~{tert}-butyl ~{N}-[(2~{S})-1-[(2~{S},4~{R})-2-[[(1~{R},2~{R})-1-(cyclopropylsulfonylcarbamoyl)-2-ethyl-cyclopropyl]carbamoyl]-4-(3-ethyl-7-methoxy-quinoxalin-2-yl)oxy-pyrrolidin-1-yl]-3,3-dimethyl-1-oxidanylidene-butan-2-yl]carbamate 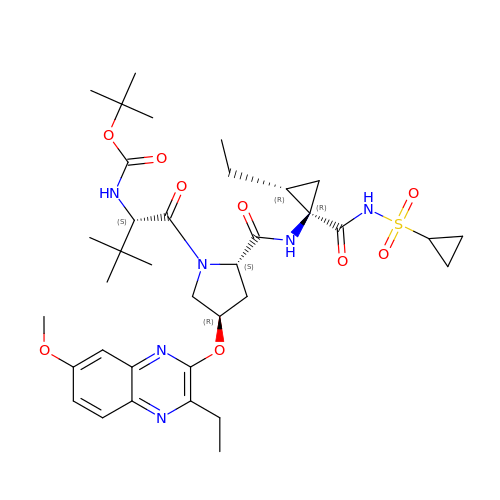| C36 H52 N6 O9 S | QHOOZSSNIATKFV-ZCNUFEDYSA-N> MTSQGDTTSGTQLKPPVEAVRSHYDKSNEFFKLWLDPSMTYSCAYFERPDMTLEEAQYAKRKLALDKLNLEPGMTLLDIGCGWGSTMRHAVAEYDVNVIGLTLSENQYAHDKAMFDEVDSPRRKEVRIQGWEEFDEPVDRIVSLGAFEHFADGAGDAGFERYDTF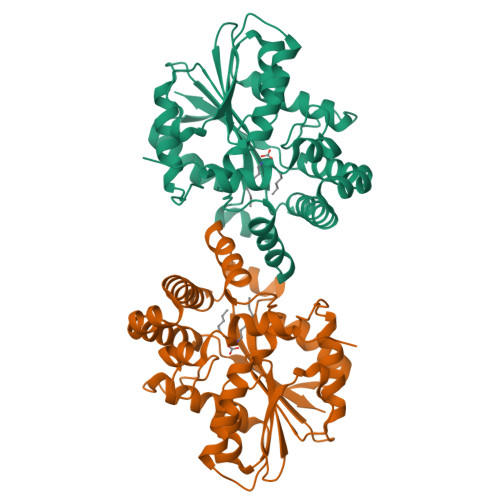FKKFYNLTPDDGRMLLHTITIPDKEEAQELGLTSPMSLLRFIKFILTEIFPGGRLPRISQVDYYSSNAGWKVERYHRIGANYVPTLNAWADALQAHKDEAIALKGQETCDIYMHYLRGCSDLFRDKYTDVCQFTLVK> MRHFRLNRCSYTPNLTSLTNQVNRSERLRKWGSAGVPPGVPRIPRLEAKGIAILHESPKV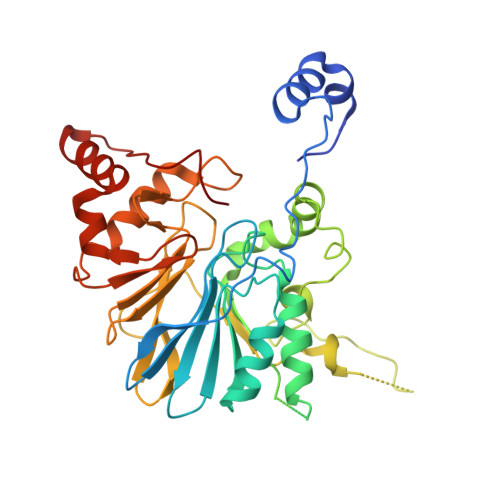ILAGRSRCNNFDSNQYMLINKATKRCLLVDASDDWPDDWAAFIGASDLTLTHVFLTHCHIDNIINLNAFLTICGSRQKQRVQVDSQDNDNREDDNGSDEIGVMWCPAEECWVQNFKRSCERYGRFEEMHQVLPMMCRSLYTPQHLVDPVIAGFSRRNARHLRRNDVLLSAATNRATSFIDFGNGVLLYYIFSPGHSPGHMMLHIPTERILFSGDLLFFNKVGRVDLPWATGVRLAESLRLLEALPDNTVVVPGHGRMTTLGRERRENKALQQCYQRQEIGKQEVSVGFNEGYL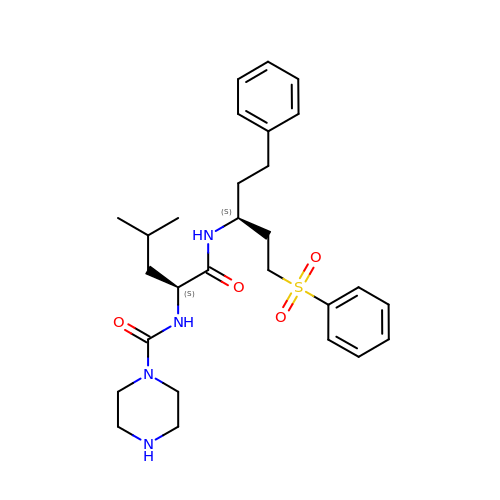N-{(1R)-3-phenyl-1-[2-(phenylsulfonyl)ethyl]propyl}-N~2~-(piperazin-1-ylcarbonyl)-L-leucinamide | C28 H40 N4 O4 S | GZQYXFWTRHRNKT-AHWVRZQESA-N In the Firmicute B. subtilis, the ytqI gene product was shown to be a major nanoRNA turnover enzyme, and was renamed NanoRNase A (NrnA). We show here that Bacillus NrnA is a bidirectional nuclease that can degrade RNA fragments from either the 3′ or the 5′ end. We have determined crystal structures of B. subtilis NrnA in its apo form, as well as complexed with substrates. These structures reveal a dynamic bi-lobed molecule with the DHH catalytic domain and the DHHA1 substrate binding domains connected through an extended linker.

To examine binding of larger nanoRNA substrates, crystallization of NrnA with several di- and tri-nucleotide ligands were carried out. In most of these trials, the substrate was likely hydrolyzed due to residual activity of the H103A mutant as no additional density was visible. However, the crystal structure of NrnA H103A:pAA*A complex (pAA*A, where * represents a phosphorothioate linkage, soaked into H103A in presence of EDTA and in the absence of metal) did reveal additional density. Electron density corresponding to a pA mononucleotide was seen in the same location as pAp in the H103A:pAp structure, but it was not continuous enough to build the full ligand. However, we did see a clear region of additional density between H284 and a solvent exposed phenylalanine from the catalytic domain (F162). F162 is structurally equivalent to W187 in Rv2873c, a residue observed to stack with the AMP adenosine at the 3′-end of a cleaved dinucleotide in a closed conformation of an Rv2873c monomer. As in the case of the H103A:pAp structure, the additional pAA*A density is seen only in two of the four monomers in the asymmetric unit. Unlike the H103A:pAp structure, the H103A:pAA*A structure is in a closed conformation, suggesting that a longer substrate may stabilize interactions between the two NrnA domains. Interestingly, ligand bound structures of NrnA crystals soaked with a 3 mer pAA*A are observed only in the closed conformation (spacing of 12.2 Å between Cα of H284 and Cα of H104), suggesting that nanoRNA substrates may facilitate interactions between the two domains. In this model, the 3′ terminal base can participate in a base stacking interaction with F162, a conserved solvent-exposed aromatic residue from the catalytic domain, as suggested by electron density observed in the H103A:pAA*A co-crystal structure.

>[4x]MGSSHHHHHHENLYFQSMASMKTELIRTISLYDTIILHRHVRPDPDAYGSQCGLTEILRETYPEKNIFAVGTPEPSLSFLYSLDEVDNETYEGALVIVCDTANQERIDDQRYPSGAKLMKIDAHPNEDPYGDLLWVDTSASSVSEMIYELYLEGKEHGWKLNTKAAELIYAGIVGDTGRFLFPNTTEKTLKYAGELIQYPFSSSELFNQLYETKLNVVKLNGFIFQNVSLSENGAASVFIKKDTLEKFGTTASEASQLVGTLGNISGIRAWVFFVEEDDQIRVRFRSKGPVINGLARKYNGGGHPLASGASIYSWDEADRILADLETLCKEHE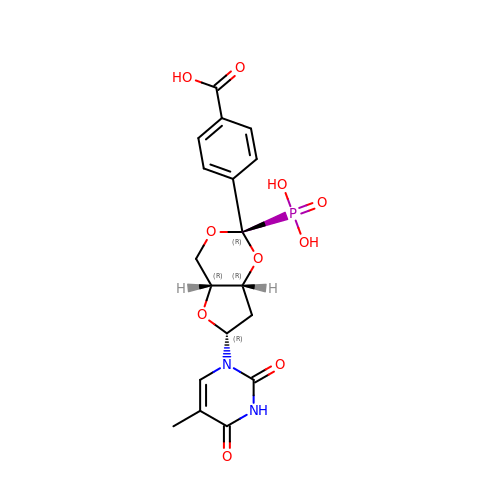1-{3,5-O-[(4-carboxyphenyl)(phosphono)methylidene]-2-deoxy-beta-D-threo-pentofuranosyl}-5-methylpyrimidine-2,4(1H,3H)-dione | C18 H19 N2 O10 P | FUFYAXRWQXEVGS-UHQDVWGKSA-N In platelets, scrambling is mediated by the protein TMEM16F, which catalyzes the externalization of phosphatidylserine (PS) in response to an increase in the intracellular Ca2+ concentration to trigger blood clotting. TMEM16F belongs to the TMEM16 protein family, whose members either function as Ca2+ activated anion-selective channels or as Ca2+ activated lipid scramblases. To better understand how the small sequence differences in TMEM16F give rise to its distinct functional properties, we determined the structure of murine TMEM16F (mTMEM16F) by cryo-EM in Ca2+-bound and Ca2+-free states, both in a detergent and in a lipid environment. By combining data from cryo-electron microscopy, in vitro scrambling assays and electrophysiology, our study has provided insight into the diverse functional behavior of mTMEM16F, a member of the TMEM16 family that facilitates the transport of lipids and ions across cellular membranes. Both processes are controlled by the binding of Ca2+ to a site located within the transmembrane domain that is accessible from the cytoplasm and they are mediated by the same structural element located at the periphery of each subunit.

For that purpose, we determined structures of mTMEM16F in the absence and presence of Ca2+. Structures of the protein in the detergent digitonin were determined for Ca2+-bound and Ca2+-free states by cryo-EM at 3.2 Å and 3.6 Å, respectively (Figure 2—figure supplements 1 and 2). The equivalence of the Ca2+-free conformation of mTMEM16F with an inactive ligand-free state of a TMEM16 scramblase is evident in the low RMSD of 2.0 Å of a superposition with the Ca2+-free conformation of nhTMEM16 in nanodiscs. The conformational changes that take place in mTMEM16F upon ligand binding can be appreciated in the comparison of Ca2+-bound and Ca2+-free conformations. As in mTMEM16A, the absence of Ca2+ causes a local transition confined to the pore region, whereas the remainder of the structure remains largely unaffected. Besides comparably small rearrangements of α3 and α4, which are less pronounced in the nanodisc structures, the largest difference is found at the intracellular half of α6 (α6c). In the ligand-free state, this helix has altered its conformation in response to the loss of the positively charged interaction partner, leading to an increase in mobility of α6c as indicated by the weaker density. The transition can be described by a rigid-body movement of α6c by 20°, around a hinge located close to a conserved glycine residue (Gly 615), whose equivalent in mTMEM16A was shown to be critical for conformational rearrangements. Thus, whereas in the apo-form of mTMEM16A α6c approaches α4, thereby closing the gap between both helices, the movement of α6c in mTMEM16F is directed away from α4.

>[2x]MQMMTRKVLLNMELEEDDDEDGDIVLENFDQTIVCPTFGSLENQQDFRTPEFEEFNGKPDSLFFTDGQRRIDFILVYEDESKKENNKKGTNEKQKRKRQAYESNLICHGLQLEATRSVSDDKLVFVKVHAPWEVLCTYAEIMHIKLPLKPNDLKTRSPFGNLNWFTKVLRVNESVIKPEQEFFTAPFEKSRMNDFYILDRDSFFNPATRSRIVYFILSRVKYQVMNNVNKFGINRLVSSGIYKAAFPLHDCRFNYESEDISCPSERYLLYREWAHPRSIYKKQPLDLIRKYYGEKIGIYFAWLGYYTQMLLLAAVVGVACFLYGYLDQDNCTWSKEVCDPDIGGQILMCPQCDRLCPFWRLNITCESSKKLCIFDSFGTLIFAVFMGVWVTLFLEFWKRRQAELEYEWDTVELQQEEQARPEYEAQCNHVVINEITQEEERIPFTTCGKCIRVTLCASAVFFWILLIIASVIGIIVYRLSVFIVFSTTLPKNPNGTDPIQKYLTPQMATSITASIISFIIIMILNTIYEKVAIMITNFELPRTQTDYENSLTMKMFLFQFVNYYSSCFYIAFFKGKFVGYPGDPVYLLGKYRSEECDPGGCLLELTTQLTIIMGGKAIWNNIQEVLLPWVMNLIGRYKRVSGSEKITPRWEQDYHLQPMGKLGLFYEYLEMIIQFGFVTLFVASFPLAPLLALVNNILEIRVDAWKLTTQFRRMVPEKAQDIGAWQPIMQGIAILAVVTNAMIIAFTSDMIPRLVYYWSFSIPPYGDHTYYTMDGYINNTLSVFNITDFKNTDKENPYIGLGNYTLCRYRDFRNPPGHPQEYKHNIYYWHVIAAKLAFIIVMEHIIYSVKFFISYAIPDVSKITKSKIKREKYLTQKLLHESHLKDLTKNMGIIAERIGGTVDNSVRPKLE>GSINMATVPVYCVCRLPYDVTRFMIECDACKDWFHGSCVGVEEEEAPDIDIYHCPNCEKTHGKSTLKKKRTWHKHGPGQAPDVKPVQNGSQLFIKELRSRTFPSAEDVVARVPGSQLTLGYMEEHGFTEPILVPKKDGLGLAVPAPTFYVSDVENYVGPERSVDVTDVTKQKDCKMKLKEFVDYYYSTNRKRVLNVTNLEFSDTRMSSFVEPPDIVKKLSWVENYWPDDALLAKPKVTKYCLICVKDSYTDFHIDSGGASAWYHVLKGEKTFYLIRPASANISLYERWRSASNHSEMFFADQVDKCYKCI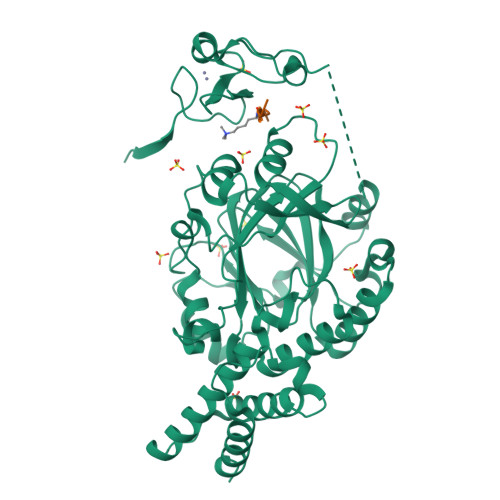VKQGQTLFIPSGWIYATLTPVDCLAFAGHFLHSLSVEMQMRAYEVERRLKLGSLTQFPNFETACWYMGKHLLEAFKGSHKSGKQLPPHLVQGAKILNGAFRSWTKKQALAEHEDELPEHFKPSQLIKDLAKEIRLSENASKAVRP[2x];>PRVKAAQAGRQS[2x]>CGTGAATTCACG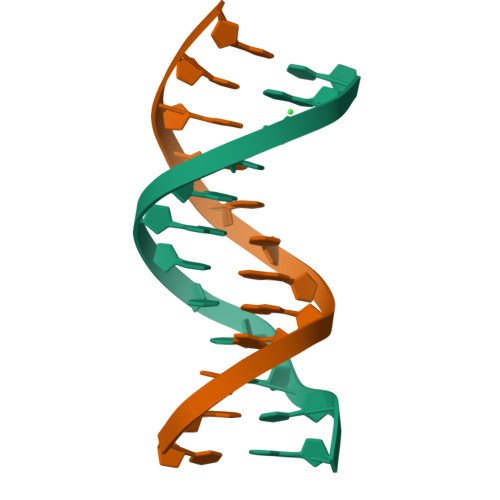[2x]>[2x]MEPQEEFITTEEVEQEIVPTVEVEQDVPVDIEGENDDDDEMMNDDE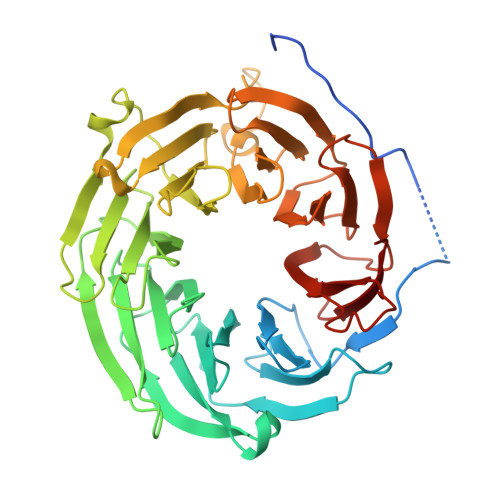EALEVDMSNNSLTYFDKHTDSVFAIGHHPNLPLVCTGGGDNLAHLWTSHSQPPKFAGTLTGYGESVISCSFTSEGGFLVTADMSGKVLVHMGQKGGAQWKLASQMQEVEEIVWLKTHPTIARTFAFGATDGSVWCYQINEQDGSLEQLMSGFVHQQDCSMGEFINTDKGENTLELVTCSLDSTIVAWNCFTGQQLFKITQAEIKGLEAPWISLSLAPETLTKGNSGVVACGSNNGLLAVINCNNGGAILHLSTVIELKPEQDELDASIESISWSSKFSLMAIGLVCGEILLYDTSAWRVRHKFVLEDSVTKLMFDNDDLFASCINGKVYQFNARTGQEKFVCVGHNMGVLDFILLHPVANTGTEQKRKVITAGDEGVSLVFEVPN> WEIDPKDLTFLKELGTGQFGVVKYGKWRGQYDVAIKMIKEGSMSEDEFIEEAKVMMNLSHEKLVQLYGVCTKQRPIFIITEYMANGCLLNYLREMRHRFQTQQLLEMCKDVCEAMEYLESKQFLHRDLAAR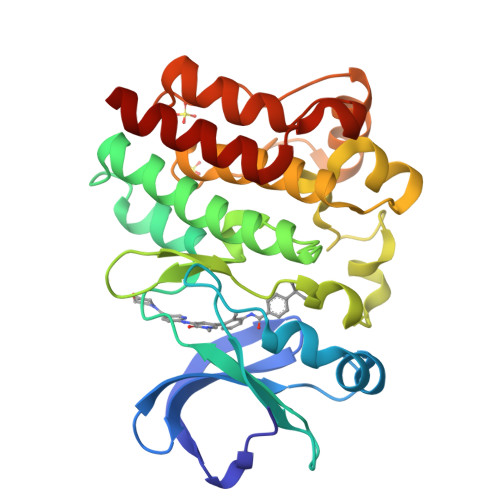NCLVNDQGVVKVSDFGLSRYVLDDEYTSSVGSKFPVRWSPPEVLMYSKFSSKSDIWAFGVLMWEIYSLGKMPYERFTNSETAEHIAQGLRLYRPHLASEKVYTIMYSCWHEKADERPTFKILLSNILDVMDEN>[2x]MGAAILPDLGTEILIPVCAVIGIAFALFQWLLVSKVKLSAVRDASPNAAAKNGYNDYLIEEEEGINDHNVVVKCAEIQNAISEGATSFLFTEYKYVGIFMVAFAILIFLFLGSVEGFSTSPQACSYDKTKTCKPALATAIFSTVSFLLGGVTSLVSGFLGMKIATYANARTTLEARKGVGKAFITAFRSGAVMGFLLAANGLLVLYIAINLFKIYYGDDWGGLFEAITGYGLGGSSMALFGRVGGGIYTKAADVGADLVGKVERNIPEDDPRNPAVIADNVGDNVGDIAG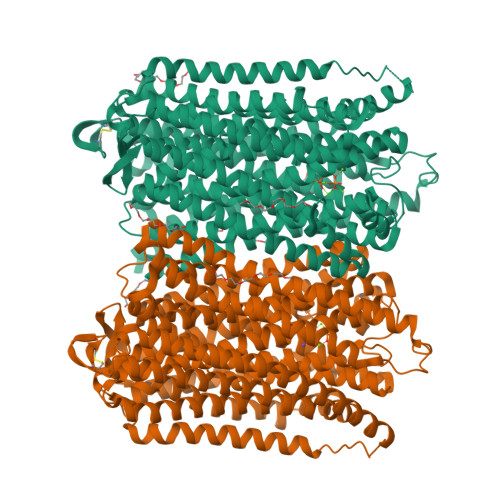MGSDLFGSYAQSSCAALVVASISSFGLNHELTAMLYPLIVSSVGILVCLLTTLFATDFFEIKAVKEIEPALKKQLVISTVLMTIGVAVVSFVALPTSFTIFNFGVQKDVKSWQLFLCVAVGLWAGLIIGFVTEYYTSNAYSPVQDVADSCRTGAATNVIFGLALGYKSVIIPIFAIAISIFVSFTFAAMYGIAVAALGMLSTIATGLAIDAYGPISDNAGGIAEMAGMSHRIRERTDALDAAGNTTAAIGKGFAIGSAALVSLALFGAFVSRASITTVDVLTPKVFIGLIVGAMLPYWFSAMTMKSVGSAALKMVEEVRRQFNTIPGLMEGTAKPDYATCVKISTDASIKEMIPPGALVMLTPLVVGILFGVETLSGVLAGSLVSGVQIAISASNTGGAWDNAKKYIEAGASEHARSLGPKGSDCHKAAVIGDTIGDPLKDTSGPSLNILIKLMAVESLVFAPFFATHGGLLFKIF>[2x]MQLFDLPLDQLQTYKPEKTAPKDFSEFWKLSLEELAKVQAEPDLQPVDYPADGVKVYRLTYKSFGNARITGWYAVPDKEGPHPAIVK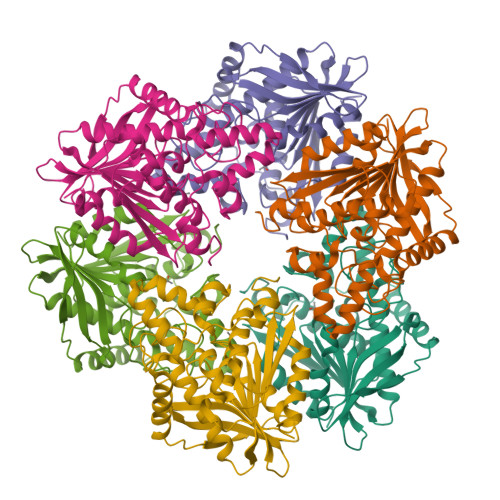YHGYNASYDGEIHEMVNWALHGYATFGMLVRGQQSSEDTSISPHGHALGWMTKGILDKDTYYYRGVYLDAVRALEVISSFDEVDETRIGVTGGAQGGGLTIAAAALSDIPKAAVADYPYLSNFERAIDVALEEPYLEINSFFRRNGSPETEVQAMKTLSYFDIMNLADRVKVPVLMSIGLIDKVTPPSTVFAAYNHLETKKELKVYRYFGHEYIPAFQTEKLAFFKQHLKG> IYGGQKAKPGDFPWQVLILGGTTAAGALLYDNWVLTAAHAVYEQKHDASALDIRMGTLKRLSPHYTQAWSEAVFIHEGYTHDAGFDNDIALIKLNNKVVINSNITPICLP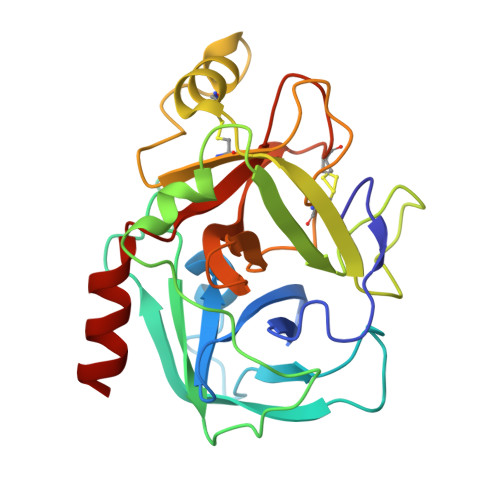RKEAESFMRTDDIGTASGWGLTQRGFLARNLMYVDIPIVDHQKCTAAYEKPPYPRGSVTANMLCAGLESGGKDSCRGDSGGALVFLDSETERWFVGGIVSWGSMNCGEAGQYGVYTKVINYIPWIENIISDF> GSHMQTPKETLSERLSALQDKIIDHYENDSKDIDSQIQYWQLIRWENAIFFAAREHGIQTLNHQVVPAYNISKSKAHKAIELQMALQGLAQSAYKTEDWTL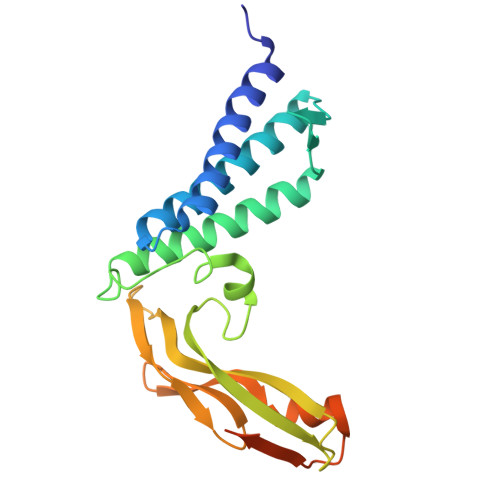QDTCEELWNTEPTHCFKKGGQTVQVYFDGNKDNCMTYVAWDSVYYMTDAGTWDKTATCVSHRGLYYVKEGYNTFYIEFKSECEKYGNTGTWEVHFGNNVIDCNDSMCSTSDDTVSAT>[4x]GSDKQEAELRRQMEGTGVEVQRQGDDIKLIMPGNITFATDSANIAPSFYAPLNNLANSFKQYNQNTIEIVGYTDSTGSRQHNMDLSQRRAQSVAGYLTAQGVD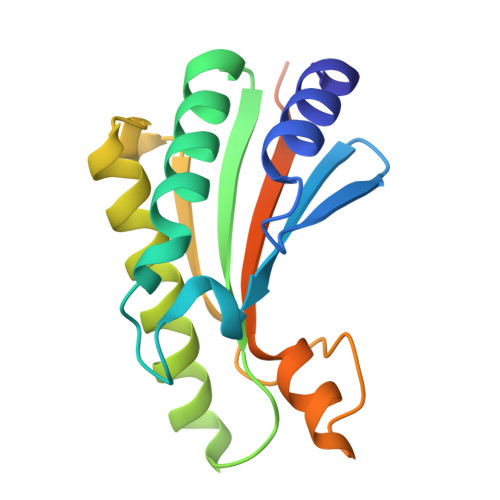GTRLSTRGMGPDQPIASNSTADGRAQNRRVEVNLRPVPGAQGPAQTQPQYGHHHHHH> YP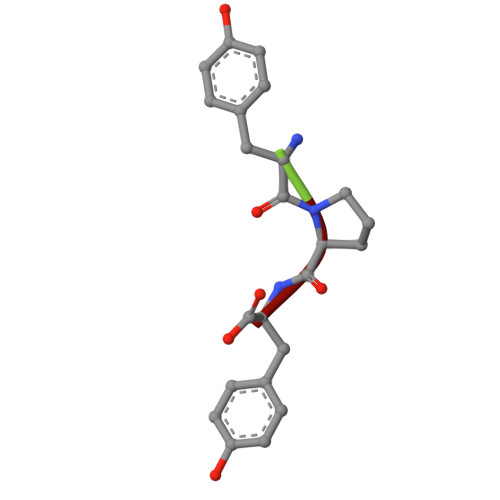Y> FR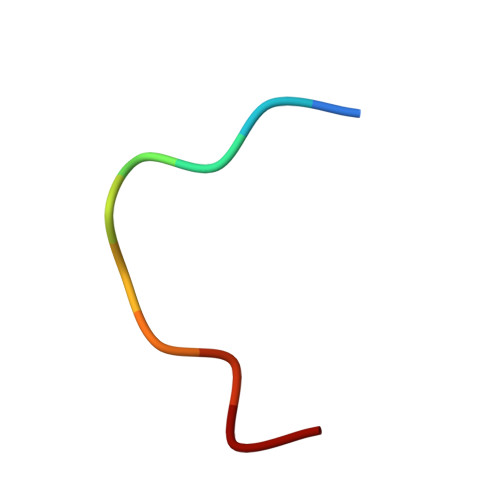SKGEELFT> TDTTNSIKHVISPLARQTLQDRDLTRPVAGKRPIRLLPWLQVVKIGGRVMDRGADAILPLVEELRKLLPEHRLLILTGAGVRARHVFSVGLDLGLPVGSLAPLAASEAGQNGHILAAMLASEGVSYVEHPTVADQLAIHLSATRAVVGSAFPPYHHHEFPGSRIPPHRADTGAFLLADAFGAAGLTIVENVDGIYTADPNGPDRGQARFLPETSATDLAKSEGPLPVDRALLDVMATARHIERVQVVNGLVPGRLTAALRGEHVGTLIRTGVRPA;> ANSTAELEELLMQRSLTDPQLQAAAAAAADFRILPDATVIKIGGQSVIDRGRAAVYPLVDEIVAARKNHKLLIGTGAGTRARHLYSIAAGLGLPAGVLAQLGSSVADQNAAMLGQLLAKHGIPVVGGAGLSAVPLSLAEVNAVVFSGMPPYKLWMRPAAEGVIPPYRTDAGCFLLAEQFGCKQMIFVKDEDGLYTANPKTSKDATFIPRISVDEM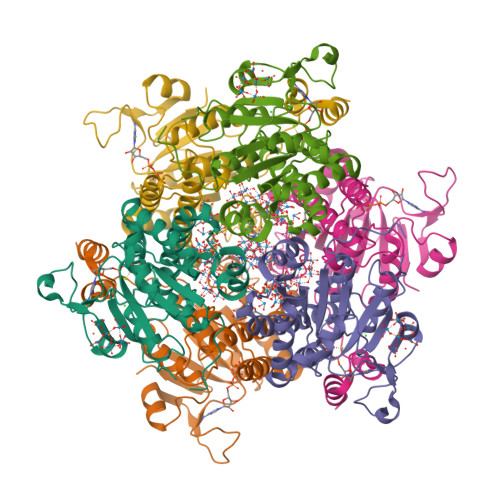KAKGLHDSILEFPVLDLLQSAQHVREVQVVNGLVPGNLTRALAGEHVGTIITAS>MKIHEFGLALFGEHYSANQFAKILINKDGSNVDRKTIQNWINRDQDLNDWVIVQLKEELLKREVILKNLLTNLSQAIMMKKLTILSKVTKDAKATAKYDESLKSGDVITYRSEDGVLLEGIISFAKKWESQRYSNLPVVEIVKLEHHHHHHH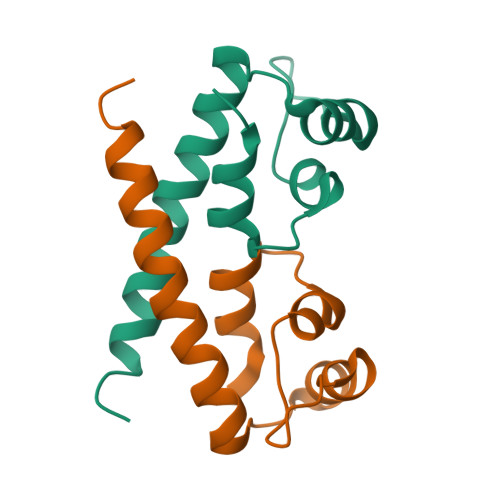H[6x]>ADSVNGAKIFSANCASCHAGGKNLVQAQKTLKKADLEKYGMYSAEAIIAQVTNGKNACPAFKGRLKPEQIEDVAAYVLGKADADWK[6x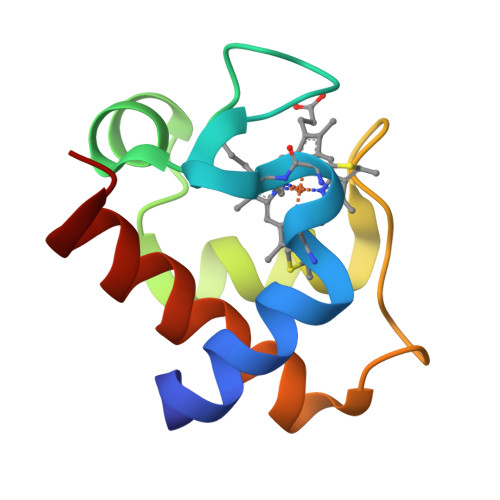]>MEDSCVLRGVMINKDVTHPRMRRYIKNPRIVLLDSSLEYKKGESQTDIEITREEDFTRILQMEEEYIHQLCEDIIQLKPDVVITEKGISDLAQHYLMRANVTAIRRVRKTDNNRIARACGARIVSRPEELREDDVG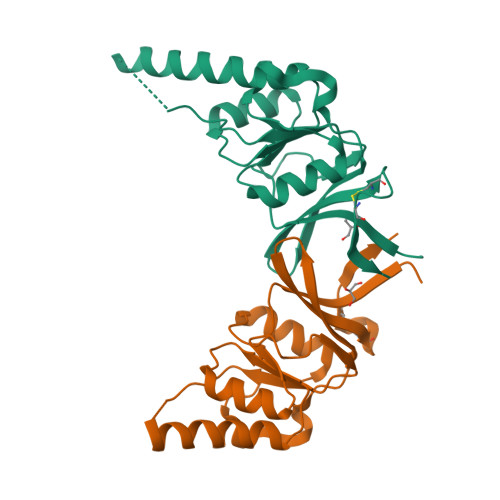TGAGLLEIKKIGDEYFTFITDCKDPKACTILLRGASHHHHHH[4x]>MQDNMMWWRGGVIYQIYPRSFLDSRGDGVGDLNGITEKLDYVASLNVDGIWLSPFFTSPMLDFGYDVSDYRDVDPMFGTLEDFKALLEKAHSLGLKVMIDQVISHTSDQHPWFQESRQNRTNPKADWFVWADPKPDGTPPNNWLSIFGGSAWTFDSRRQQYYLHNFLTSQPDVNFHHPEARQAQLDNMRFWLDLGVDGFRLDTVNFYFHDAELRDNPPVPKGEAKTLGAPEANPYTWQRHVYDLSRPENLDFLKDL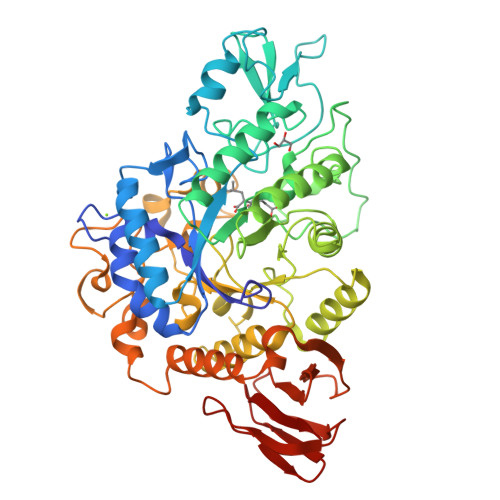RALMDEYPGTTTVGEIGDDNPLERMAEYTAGGDKLHMAYTFDLLNMPHSASYLREVIERFQRLAGDAWPCWATSNHDVVRSATRWGADEDPHAYPKVMLAVLFSLRGSVCLYQGEELGLPEADVPFERIQDPYGKVLWPEFKGRDGCRTPMPWTDGEQGGFSPVEPWLPMEARHLELAVSRQQDDPNATLNTVRALLAFRRSHPALFDGDLSLVDVGDDLLGFTRQKGDETLLCVFNLTGQEQQTTLPVEVASDLPVAHFTATRDGSTLTLPAYQAAFMQVA[2x]> GPMPMQMFMQVYDEIQMFLLEELELKFDMDPNRVRYLRKMMDTTCLGGKYNRGLTVIDVAESLLSLSPNNNGEEDDGARRKRVLHDACVCGWMIEFLQAHYLVEDDIMDNSVTRRGKPCWYRHPD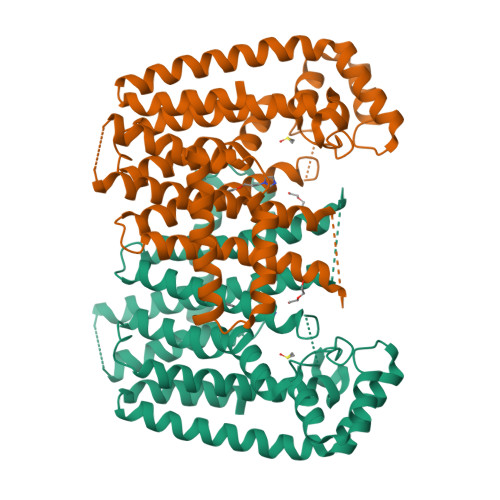VTVQCAINDGLLLKSWTHMMAMHFFADRPFLQDLLCRFNRVDYTTAVGQLYDVTSMFDSNKLDPDVSQPTTTDFAEFTLSNYKRIVKYKTAYYTYLLPLVMGLIVSEALPTVDMGVTEELAMLMGEYFQVQDDVMDCFTPPERLGKVGTDIQDAKCSWLAVTFLAKASSAQVAEFKANYGSGDSEKVATVRRLYEEADLQGDYVAYEAAVAEQVKELIEKLRLCSPGFAASVETLWGKTYKRQK> VYEKDEGQKEQLERILRQSFLFNSLDEKDLNTVILAMQEKKIEASTCLIREGDDGECLYIVQSGELNCSKLIDGEERVVKVVGPGDAFGELALLYNAPRAATVTSVSACDLWELGRDTFN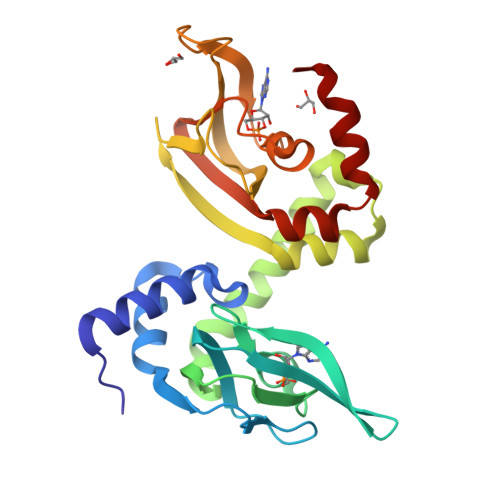AIVKDAATKRRSMYDSFLKSVHILDGMDAYERGKVADALRTEMFTDGAYIVRQGELGDVFYIVEEGSAVATKSFGPGQPPIEVKKYQAGDYFGELALINEEPRAANVIAHGICKVACLERKSFKRLMGSVQDLLSKKASEY>MSQPRTPEQALDTPGDCPPGRRDEDAGEGIQCSQRMLSFSDALLSIIATVMILPVTHTEISPEQQFDRSVQRLLATRIAVYLMTFLIVTVAWAAHTRLFQVVGKTDDTLALLNLACMMTITFLPYTFSLMVTFPDVPLGIFLFCVCVIAIGVVQALIVGYAFHFPHLLSPQIQRSAHRALYRRHVLGIVLQGPALCFAAAIFSLFFVPLSYLLMVTVILLPYVSKVTGWCRDRLLGHREPSAHPVEVFSFDLHEPLSKERVEAFSDGVYAIVATLLILDICEDNVPDPKDVKERFSGSLVAALSATGPRFLAYFGSFATVGLLWFAHHSLFLHVRKATRAMGLLNTLSLAFVGGLPLAYQQTSAFARQPRDELERVRVSCTIIFLASIFQLAMWTTALLHQAETLQPSVWFGGREHVLMFAKLALYPCASLLAFASTCLLSRFSVGIFHLMQIAVPCAFLLLRLLVGL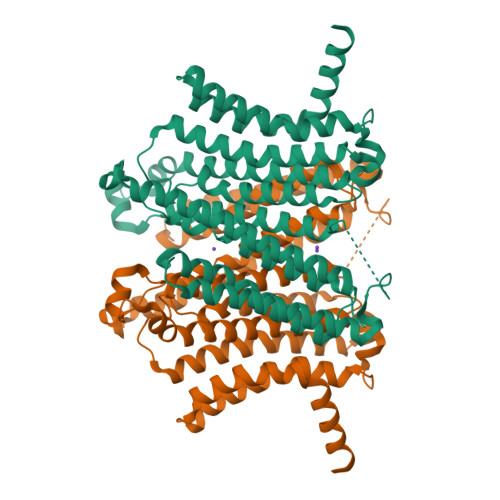ALATLRVLRGLARPEHPPPAPTGQDDPQSQLLPAPC[2x]>MTENFFGKTLAARPVEAIPGMLEFDIPVHGDNRGWFKENFQKEKMLPLGFPESFFAEGKLQNNVSFSRKNVLRGLHAEPWDKYISVADGGKVLGTWVDLREGETFGNTYQTVIDASKSIFVPRGVANGFQVLSDFVAYSYLVNDYWALELKPKYAFVNYADPSLDIKWENLEEAEVSEADENHPFLKDVKPLRK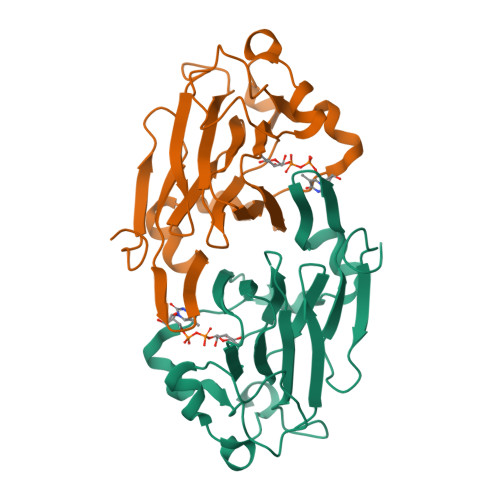EDL[4x]> MLTQEQDQQLVERVQRGDKRAFDLLVLKYQHKILGLIVRFVHDAQEAQDVAQEAFIKAYRALGNFRGDSAFYTWLYRIAINTAKNHLVARGRRPPDSDVTA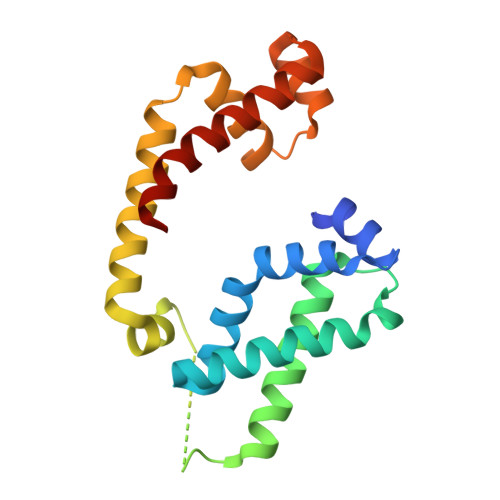EDAEFFEGDHALKDIESPERAMLRDEIEATVHQTIQQLPEDLRTALTLREFEGLSYEDIATVMQCPVGTVRSRIFRAREAIDKALQPLLREA>[2x]GAPRSHEVPLLVTLEELYLGKRKKIKVTRKRFIEHKVRNEENIVEVEIK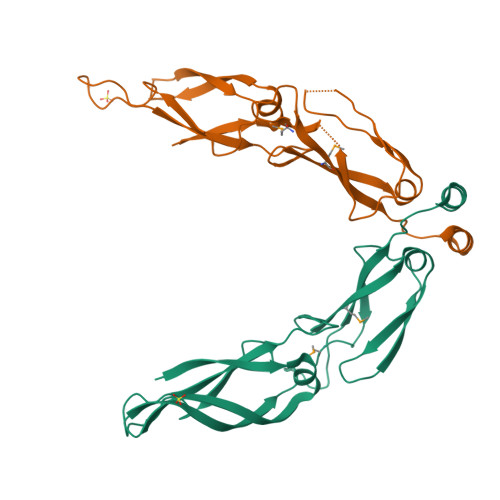PGWKDGTKLTYSGEGDQESPGTSPGDLVLIIQTKTHPRFTRDDCHLIMKVTIPLVRALTGFTCPVTTLDNRNLQIPIKEIVNPKTRKIVPNEGMPIKNQPGQKGDLILEFDICFPKSLTPEQKKLIKEALD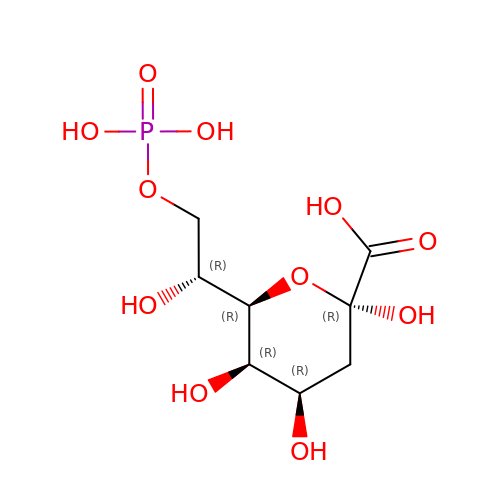3-deoxy-8-O-phosphono-alpha-D-manno-oct-2-ulopyranosonic acid | C8 H15 O11 P | IZZNRKJLBIYBJN-HXUQBWEZSA-N> MAEKFDHLEEHLEKFVENIRQLGIIVSDFQPSSQAGLNQKLNFIVTGLQDIDKCRQQLHDITVPLEVFEYIDQGRNPQLYTKECLERALAKNEQVKGKIDTMKKFKSLLIQEL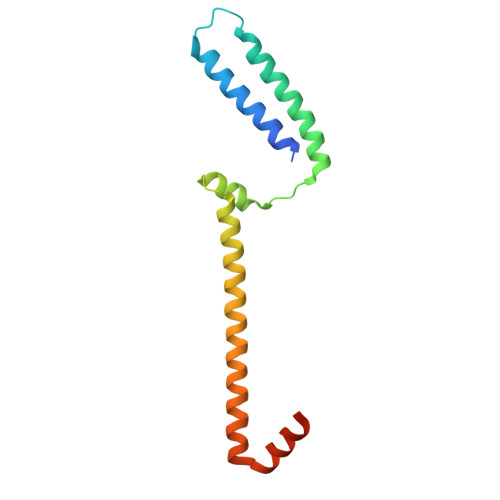SKVFPEDMAKYRSIRGEDHPPS>[2x]MLKQPIQAQQLIELLKVHYGIDIH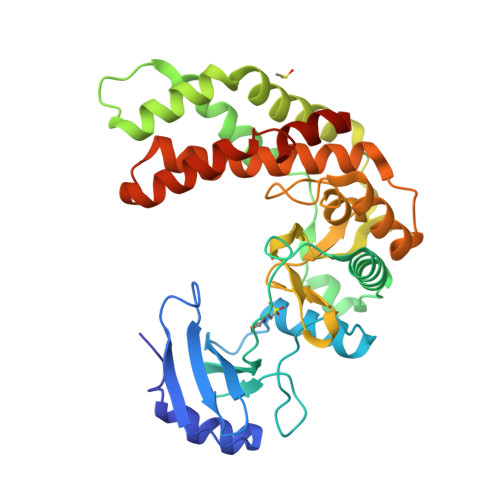TAQFIQGGADTNAFAYQADSESKSYFIKLKYGYHDEINLSIIRLLHDSGIKEIIFPIHTLEAKLFQQLKHFKIIAYPFIHAPNGFTQNLTGKQWKQLGKVLRQIHETSVPISIQQQLRKEIYSPKWREIVRSFYNQIEFDNSDDKLTAAFKSFFNQNSAAIHRLVDTSEKLSKKIQPDLDKYVLCHSDIHAGNVLVGNEESIYIIDWDEPMLAPKERDLMFIGGGVGNVWNKPHEIQYFYEGYGEINVDKTILSYYRHERIVEDIAVYGQDLLSRNQNNQSRLESFKYFKEMFDPNNVVEIAFATEQLEHHHHHH> SGVDDDMACHKIPVE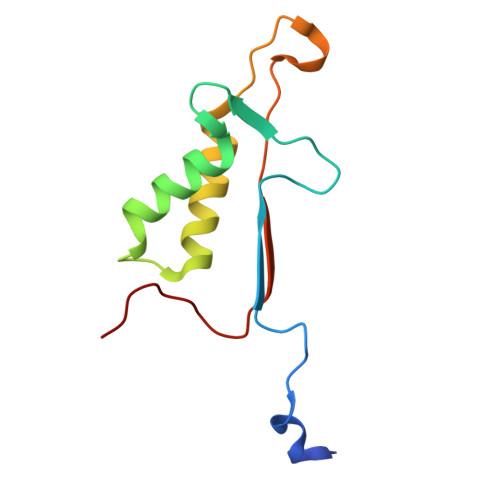ADFLYAYSTAPGYYSWRNSKDGSWFIQSLCAMLKQYADKLEFMHILTRVNRKVATEFESFSFDATFHAKKQIPCIVSMLTKELYFYHH>KVTMNDFDYLKLLGKGTFGKVILVREKATGRYYAMKILRKEVIIAKDEVAHTVTESRVLQNTRHPFLTALKYAFQTHDRLCFVMEYANGGELFFHLSRERVFTEERARFYGAEIVSALEYLHSRDVVYRDIKLENLMLDKDGHIKITD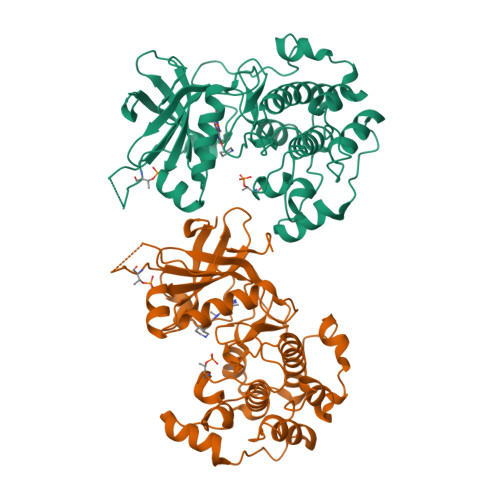FGLCKEGISDGATMKTFCGTPEYLAPEVLEDNDYGRAVDWWGLGVVMYEMMCGRLPFYNQDHERLFELILMEEIRFPRTLSPEAKSLLAGLLKKDPKQRLGGGPSDAKEVMEHRFFLSINWQDVVQKKLLPPFKPQVTSEVDTRYFDDEFTAQSITITPPDRYDSLGLLELDQRTHFPQFDYSASIR[2x]>[2x]HHHHHHFNLPPGNYKKPKLLYCSNGGHFLRILPDGTVDGTRDRSDQHIQLQLSAESVGEVYIKSTETG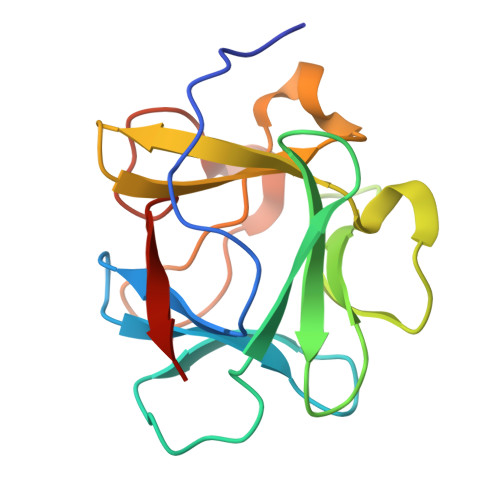QYLAMDTDGLLYGSQTPNEETLFLERLEENHYNTYISKKHAEKNWFVGLKKNGSCKRGPRTHYGQKAILFLPLPVSSD>[2x]MAHHHHHHMTTYTLVLLRHGESTWNKENKFTGWTDVPLSEKGEEEAIAAGKYLKEKNFKFDVVYTSVLKRAICTAWNVLKTADLLHVPVVKTWRLNERHYGSLQGLNKSETAKKYGEEQVKIWRRSYDIPPPKLDKEDNRWPGHNVVYKNVPKDALPFTECLKDTVERVLPFWFDHIAPDIL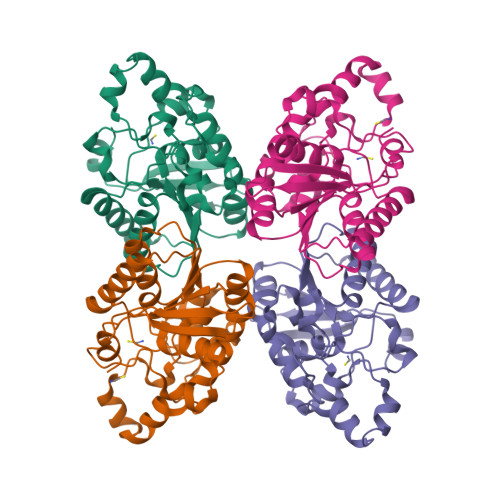ANKKVMVAAHGNSLRGLVKHLDNLSEADVLELNIPTGVPLVYELDENLKPIKHYYLLDSEELKKKMDEVANQGKAK>GMKHFLTLRDFSKEEILSLVNHASELKKEPKKLLQDKTLAMIFEKNSTRTRMAFELAITELGGKALFLSSNDLQLSRGEPVKDTARVIGAMVDFVMMRVNKHETLLEFARYSKAPVINALSELYHPTQVLGDLFTIKEWNKMQNGIAKVAFIGDSNNMCNSWLITAAILGFEISIAMPKNYKISPEIWEFAMKQALISGAKISLGYDKFEALKDKDVVITDTWVSMGEENEKERKIKEFEGFMIDEKAMSVANKDAILLHCLPAYRGYEVSEEIFEKHADVIFEEARNRLYVVKA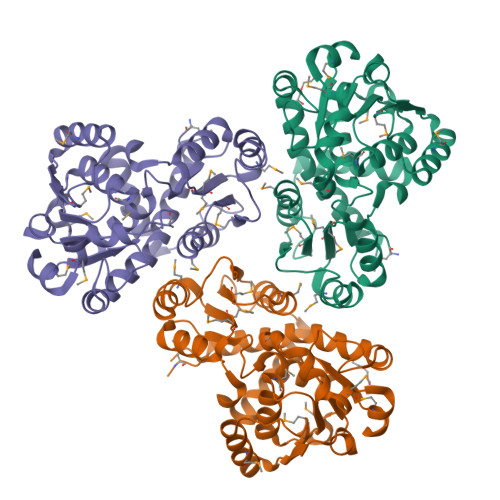LLCFLDNQRGRE[6x]> GPLGSFKIYQQKSFEQKIESLKKEKDDQLSEGNQKEHFRQGQAEVIAYYPLQGEKVISSVRELINQDVKDKLESKDNLVFYYTEQEESGLKGVVNRNVTKQIYDLVAFKIEETEKTSLGKVHLTEDGQPFTLDQLFSDASKAKEQLIKELTSFIEDKKIEQDQSEQIVKNFSDQDLSAWNFDYKDSQIILYPSPVVENLEEIALPVSAFFDVIQSSYLLEKDAALYQSYFDKKHQKVVALTFDDGPNPATTPQVLETLAKYDIKATFFVLGKNVSGNEDLVKRIKSEGHVVGNHSWSHPILSQLSLDEAKKQITDTEDVLTKVLGSSSKLMRPPYGAITDDIRNSLDLSFIMWDVDSLDWKSKNEASILTEIQHQVANGSIVLMHDIHSPTVNALPRVIEYLKNQGYTFVT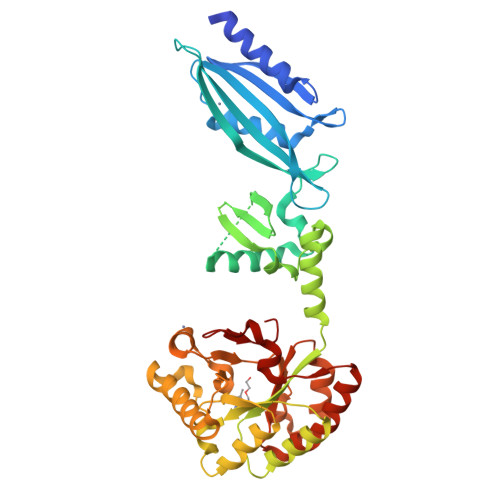IPEMLNTRLKAHELYYSRDE>MSHSKQALADTMKMTWLMEGSVNGHAFTIEGEGTGKPYEGKQSGTFRVTKGGPLPFAFDIVAPTLKYGFKCFMKYPADIPDYFKLAFPEGLTYDRKIAFEDGGCATATVEMSLKGNTLVHKTNFQGGNFPIDGPVMQKRTLGWEPTSEKMTPCDGIIKGDTIMYLMVEGGKTLKCRYENNYRANKPVLMPPSHFVDLRLTRTNLDKEGLAFKLEE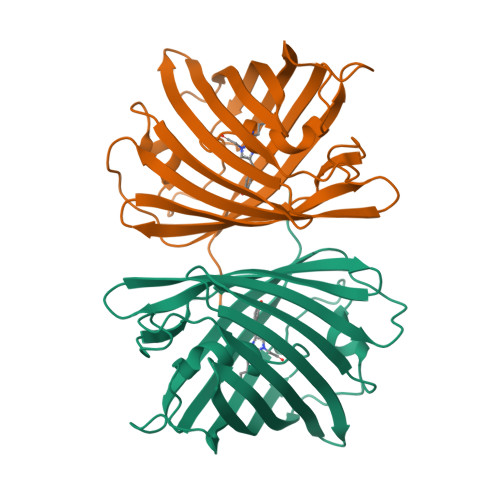YAVARVLEV[4x]> QDNSRYTHFLTQHYDAEPQGRDDRYCESIMRRRGLTSPCKDINTFIHGNKRSIKAICENKNGNPHRENLRISKSSFQVTTCK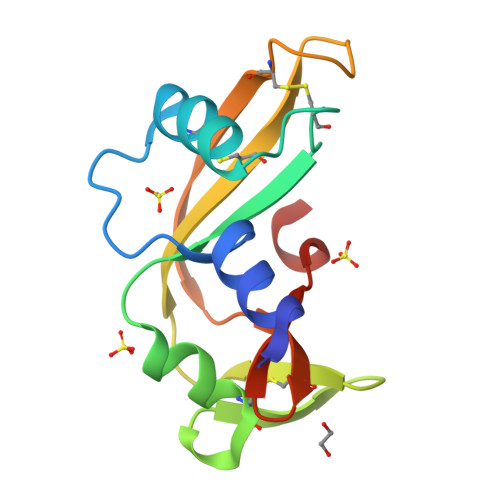LHGGSPWPPCQYRATAGFRNVVVACENGLPVHLDQSIFRRP> MLEQPYLDLAKKVLDEGHFKP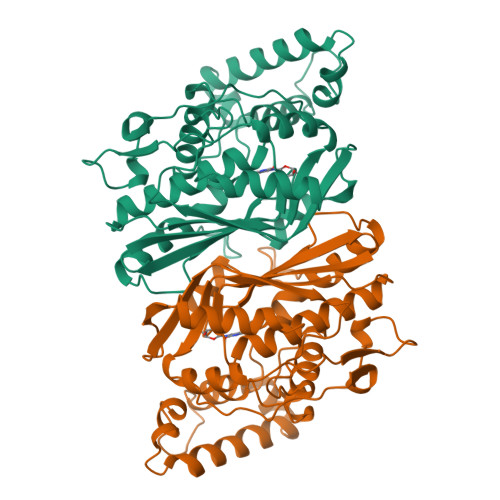DRTHTGTYSIFGHQMRFDLSKGFPLLTTKKVPFGLIKSELLWFLHGDTNIRFLLQHRNHIWDEWAFEKWVKSDEYHGPDMTDFGHRSQKDPEFAAVYHEEMAKFDDRVLHDDAFAAKYGDLGLVYGSQWRAWHTSKGDTIDQLGDVIEQIKTHPYSRRLIVSAWNPEDVPTMALPPCHTLYQFYVNDGKLSLQLYQRSADIFLGVPFGIASYALLTHLVAHECGLEVGEFIHTFGDAHLYVNHLDQIKEQLSRTPRPAPTLQLNPDKHDIFDFDMKDIKLLNYDPYPAIKAPVAV>AGAGAAGUUCUUCUC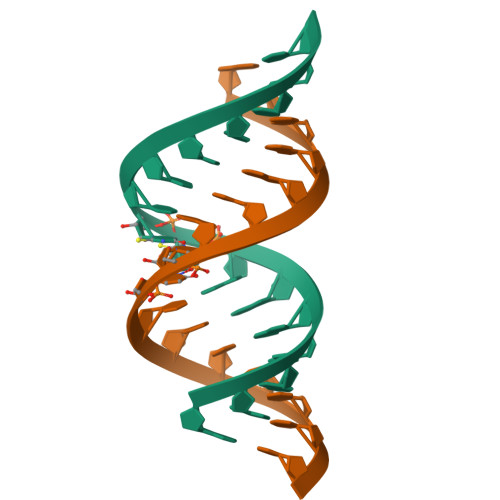U[2x]[(2~{S})-3-[[(2~{S})-1-azanyl-4-methyl-1-oxidanylidene-pentan-2-yl]amino]-2-[(3,5-diphenylphenyl)methyl]-3-oxidanylidene-propyl]-[(1~{R})-1-azanyl-3-phenyl-propyl]phosphinic 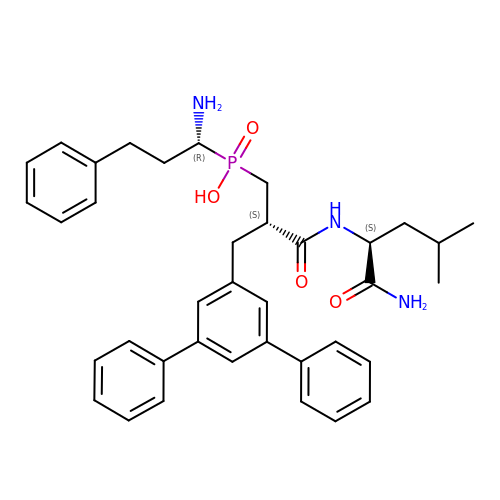acid | C37 H44 N3 O4 P | RAXDQSLZABPHNA-GVBYMILNSA-N N-[2-(2,4-diaminopyrido[2,3-d]pyrimidin-7-yl)-2-methylpropyl]-4-phenoxybenzamide | C24 H24 N6 O2 | 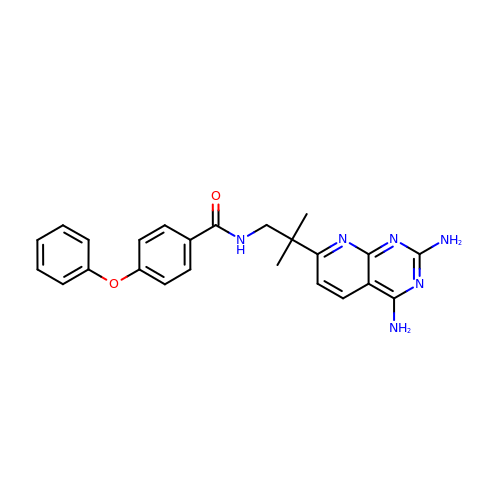FDJWFDQRPKKBFA-UHFFFAOYSA-N>[3x]NKGSIEGREPAVYFKEQFLDGDGWTSRWIESKHKSDFGKFVLSSGKFYGDEEKDKGLQTSQDARFYALSASFEPFSNKGQTLVVQFTVKHEQNIDCGGGYVKLFPNSLDQTDMHGDSEYNIMFGPDICGPGTKKVHVIFNYKGKNVLINKDIRCKDDEFTHLYTLIVRPDNTYEVKIDNSQVESGSLEDD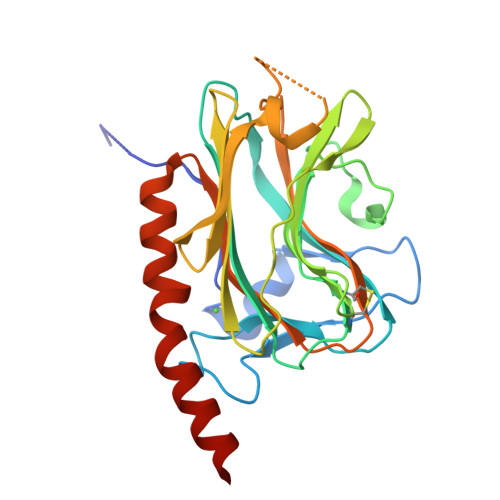WDFLPGSGDPSIYAYDNFGVLGLDLWQVKSGTIFDNFLITNDEAYAEEFGNETWGVTKAAEKQMKDKQDEEQRLK>MMNEKILIVDDQSGIRILLNEVFNKEGYQTFQAANGLQALDIVTKERPDLVLLDMKIPGMDGIEILKRMK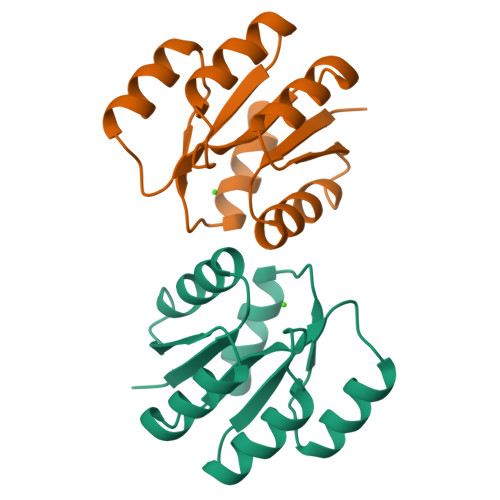VIDENIRVIIMTAYGELDMIQESKELGALTHFAKPFDIDEIRDAVKKYLPLKSN[3x]>[4x]GSHMTNDIYFMTLAIEEAKKAAQLGEVPIGAIITKDDEVIARAHNLRETLQQPTAHAEHIAIERAAKVLGSWRLEGCTLYVTLEPCVMCAGTIVMSRIPRVVYGADDPK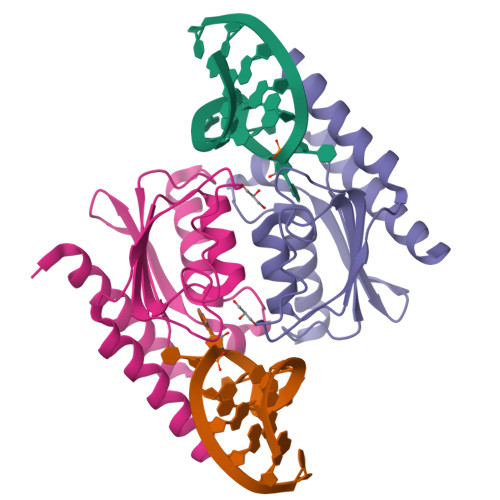GGCSGSLMNLLQQSNFNHRAIVDKGVLKEACSTLLTTFFKNLRANKKSTN> AKPDRSSFVPSLFSKKKKNVTMRSIKTTRDRVPTYQYNMNFEKLGKCIIINNKNFDKVTGMGVRNGTDKDAEALFKCFRSLGFDVIVYNDCSCAKMQDLLKKASEEDHTNAACFACILLSHGEENVIYGKDGVTPIKDLTAHFRGDRCKTLLEKPKLFFIQACRGTELDDGIQADSGPINDTDANPRYKIPVEADFLFAYSTVPGYYSWRSPGRGSWFVQALCSILEEHGKDLEIMQILTRVNDRVARH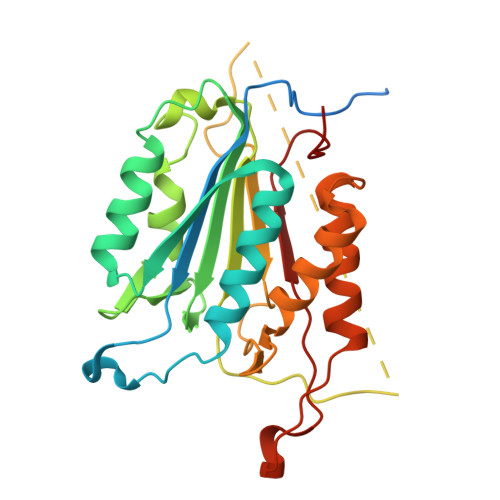FESQSDDPHFHEKKQIPCVVSMLTKELYFSQ> MLLWRRCRAWLEIRRLDKELAQSSGLPLE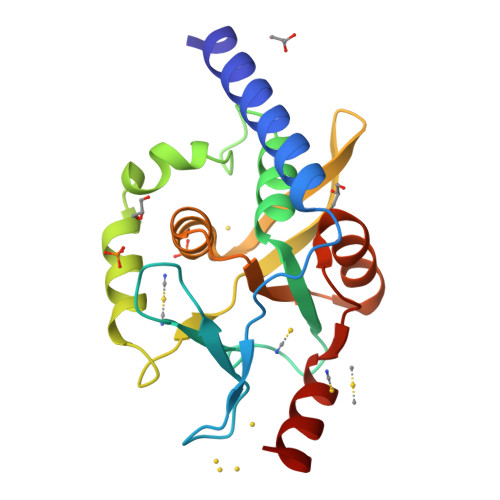LPQIVPNAWNEVVWRLPVPNHPDAFMTASNAAQSDFIVYVNGLAFYRAWLALGVEDSQACPLKQDMPKDRKYPSSAAHFAVGIDSPVPLADVSPTMILGHFAVCFTDGMTRSMWLLAHEVAVFPVLSRDEASAVMLAEHVGVAAPIQVSKLREQCRKIL> SKDELQVLLHDLELKLLQNITHHITVTGQAPTSEAIVSAVNQAGISGITEAQAHIIVNNALKLYSQDKTGMVDFALESGGGSILSTRCSETYETKTALLSLFGVPLWYFSQSPRVVIQPDIYPGNCWAFKGSQGYLVVRLSMKIYPTTFTMEHIPKTLSPTGNISSAPKDFAVYGLETEYQEEGQPLGRFTYDQEGDSLQMFHTLERPDQAFQIVELRVLSNWGHPEYTCLYRFRVHGE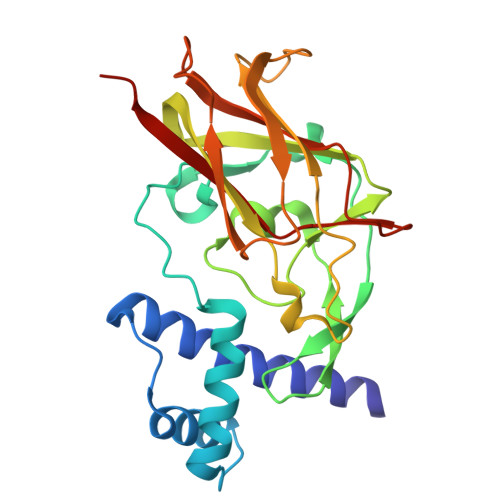PIQ>MRGSHHHHHHGSWETEERPRTREEECHFYAGGQVYPGEASRVSVADHSLHLSKAKISKPAPYWEGTAVIDGEFKELKLTDYRGKYLVFFFYPLDFTFVCPTEIIAFGDRLEEFRSINTEVVACSVDSQFEHLAWINTPRRQGGLGPIRIPLLSDLTHQISKDYGVYLEDSGHTLRGLFIIDDKGILRQITLNDLPVGRSVDETLRLVQAFQYTDKH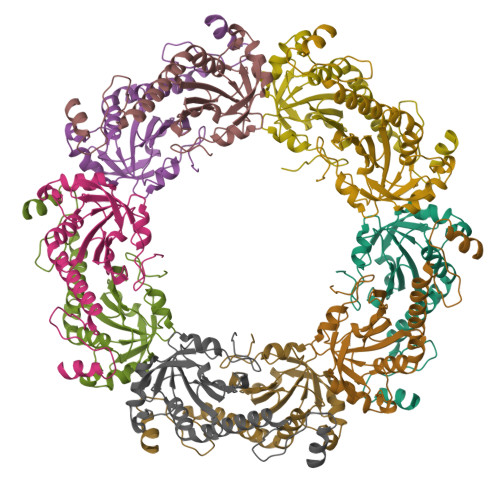GEVCPAGWKPGSETIIPDPAGKLKYFDKLN[10x]>[8x]MNAQAEEFKKYLETNGIKPKQFHKKELIFNQWDPQEYCIFLYDGITKLTSISENGTIMNLQYYKGAFVIMSGFIDTETSVGYYNLEVISEQATAYVIKINELKELLSKNLTHFFYVFQTL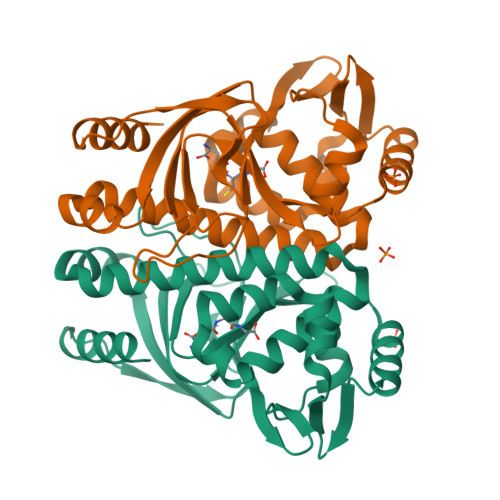QKQVSYSLAKFNDFSINGKLGSICGQLLILTYVYGKETPDGIKITLDNLTMQELGYSSGIAHSSAVSRIISKLKQEKVIVYKNSCFYVQNLDYLKRYAPKLDEWFYLACPATWGKLN>KAINNIVASFSSVNDAITQTAEAIHTVTIALNKIQDVVNQQGSALNHLTSQLRHNFQSGGRGSGRGGNLT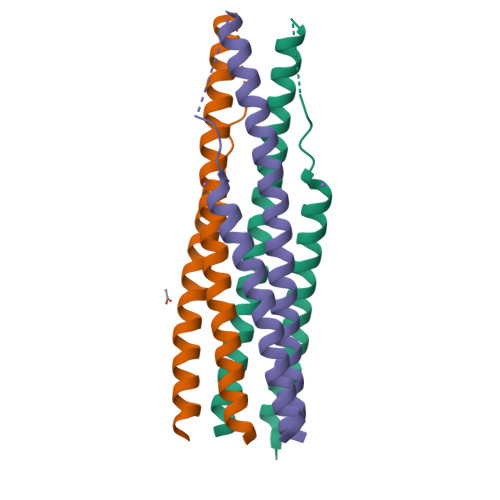YLNLSSELKQLEAKTASLFQTTVELQGLIDQINSTYVDL[3x]> MTFKAPDSLAEQIAHHLAERIIRGELKERERIQEQKVTQTLNVSRGSVREALLILERRHLVNILPRRGAQVSELSPQHVESLYALIVQLYILLAESVARRWRSEAELAPFLVIQQRLLNNLAQSDIDGFVEASFDIMRAAFPFANNPYLQETVENLLPAVSRAYHLALERRKAEMNQFLGSFAQLLQAVIARDEARIREVLLEYGRHNCQLVLAALAER

In this study, we identified a GntR/VanR transcription regulator AlkR of Pseudomonas aeruginosa SJTD‐1 involved in the negative regulation of AlkB2 and deciphered its nature of DNA binding and ligand release. The dimer of AlkR recognizes and binds to a conserved palindromic motif in the promoter of the alkB2 gene, and structural symmetry is vital for DNA binding and transcription repression. The long‐chain fatty acyl coenzyme A compounds can release AlkR and stimulate transcription of alkB2, reflecting the effect of alkane catabolic metabolites. Structural insights unveiled that the arginine residues and scaffold residues of AlkR are critical for DNA binding.

The asymmetric unit of the structure comprises a dimer of AlkR, with each monomer featuring an N‐terminal DNA binding domain (residues 1–71) and a C‐terminal effector binding domain (residues 76–219). The DNA binding domain of AlkR protein is characterized by the presence of two β‐strands (β1 and β2) and three α‐helices (α1 to α3). The helix–turn–helix motif, formed by α2 and α3, is linked to the anti‐parallel β‐strands (β1 and β2) via a small loop (wing motif). The C‐terminal domain contributes to the secondary structure of AlkR protein with six additional helices (α4 to α9), which are indicative of AlkR protein classification within the VanR‐group regulators belonging to the FCD subfamily of the GntR superfamily. A chemical cross‐linking assay with sulfo‐EGS showed that AlkR protein is predominantly in the dimer form in solution, consistent with the results of size exclusion chromatography. In this work, the Apo‐form structure of AlkR dimers revealed that the Arg45 and Arg49 are involved in interactions with the major groove of DNA, by forming hydrogen bonds with specific DNA bases. This interaction is likely pivotal for the recognition and binding of AlkR protein to its specific DNA motif, and removal of the side chains of arginine resulted in the decreased DNA affinity of AlkR protein. Moreover, a flexible sequence (specifically at residues 64–67) in the N‐terminal of AlkR is also important for its DNA binding, predominantly interacting with the minor groove of the DNA helix. Specifically, residues I63 and G68 in AlkR protein are situated on the linker of the flexible minor groove insertion sequence, potentially acting as a scaffold of this region for stabilization by hydrogen bonding via their side chains. The structural modeling results of AlkR protein and C18‐CoA using AutoDock revealed that C18‐CoA was surrounded by the C‐terminal effector‐binding domain of AlkR protein composed of helices α4‒α9.>MQTKLTIWCSEKQVDILQKLGEEFKAKYGIPVEVQYVDFGSIKSKFLTAAPQGQGADIIVGAHDWVGELAVNGLIEPIPNFSDLKNFYDTALKAFSYGGKLYGVPYAMEAVALIYNKDYVDSVPKTMDELIEKAKQIDEEYGGEVRGFIYDVANFYFSAPFILGYGGYVFKETPQGLDVTDIGLANEGAVKGAKLIKRMIDEGVLTPGDNYGTMDSMFKEGLAAMIINGLWAIKSYKDAGINYGVAPIPELEPGVPAKPFVGVQGFMINAKSPNKVIAMEFLTNFIARKETMYKIYLADPRLPARKDVLELVKDNPDVVAFTQSASMGTPMPNVPEMAPVWSAMGDALSIII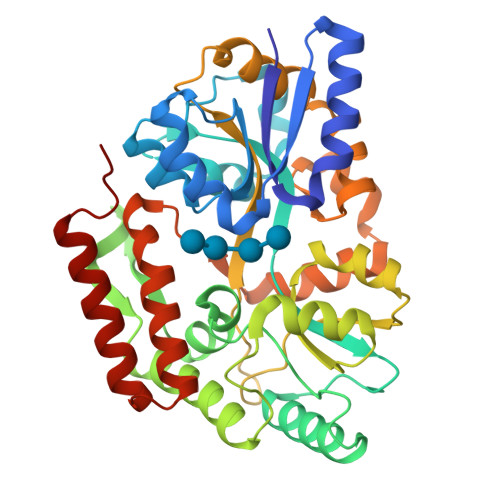NGQASVEDALKEAVEKIKAQIEKGSHHHHHH[2x]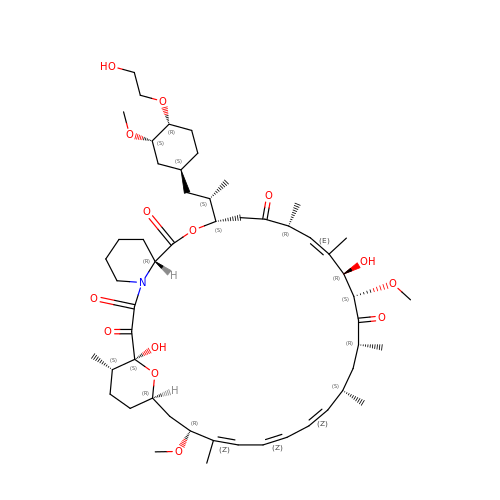Everolimus | C53 H83 N O14 | HKVAMNSJSFKALM-PGYDAPRHSA-N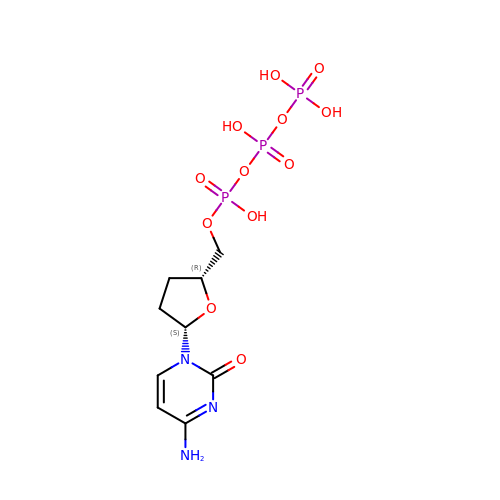[[(2~{R},5~{S})-5-(4-azanyl-2-oxidanylidene-pyrimidin-1-yl)oxolan-2-yl]methoxy-oxidanyl-phosphoryl] phosphono hydrogen phosphate | C9 H16 N3 O12 P3 | ARLKCWCREKRROD-SVRRBLITSA-N> GAASKKVNVLVVGLDNSGKTTIIERLKPRPRQAAEVAPTVGFTVDEVEKGPLTFTVFDMSGAGRYRTLWEQYYREADAVVFVVDSADKLRMVVARDEMEHMLKHSNMRKVPILYFANKKD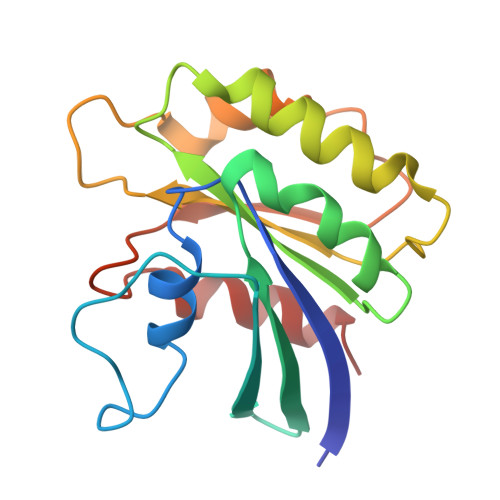LPVAMPPVEIAQALGLDDIKDRPWQIVPSNGLTGEGVDKGIDWLAERLS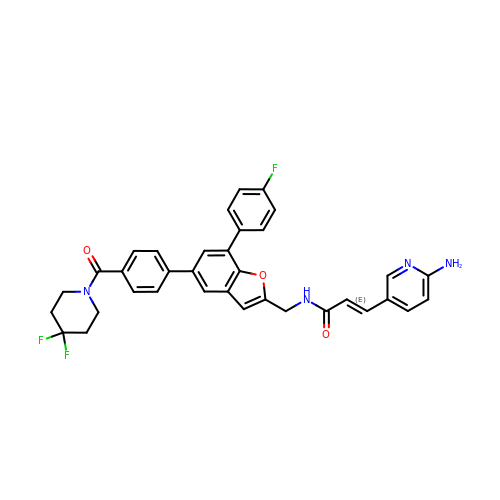(~{E})-3-(6-azanylpyridin-3-yl)-~{N}-[[5-[4-[4,4-bis(fluoranyl)piperidin-1-yl]carbonylphenyl]-7-(4-fluorophenyl)-1-benzofuran-2-yl]methyl]prop-2-enamide | C35 H29 F3 N4 O3 | MRFOPLWJZULAQD-SWGQDTFXSA-N> AQTVPYGIPLIKADKVQAQGFKGANVKVAVLDTGIQASHPDLNVVGGASFVAGEA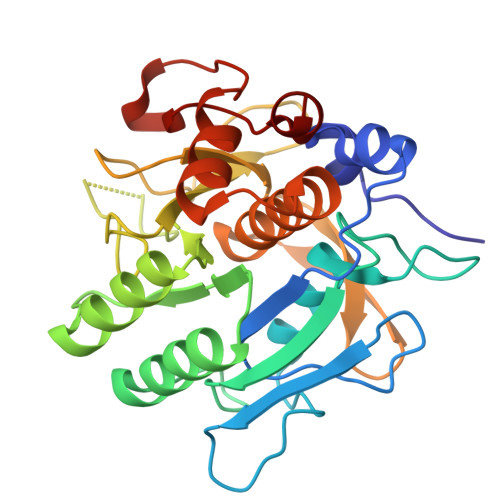YNTDGNGHGTHVAGTVAALDNTTGVLGVAPSVSLYAVKVLNSSGSGSYSGIVSGIEWATTNGMDVINMSLGGASGSTAMKQAVDNAYARGVVVVAAAGNSGSSGNTNTIGYPAKYDSVIAVGAVDSNSNRASFSSVGAELEVMAPGAGVYSTYPTNTYATLNGTSMASPHVAGAAALILSKHPNLSASQVRNRLSSTATYLGSSFYYGKGLINVEAAAQ> MLQQPTGGYTTLEQFAFTIRNDGTNATPTQFLQLLSWEATENELVKKTIPTPETHLPSARNVPGNVYIEDAITQAL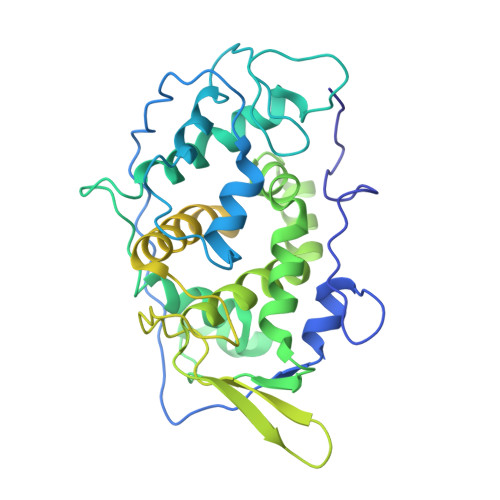FGISAQNVNAHGYFSRLSALALPNTSARLGLDGVIYNSETINIPFYDPAAVANFAATYAKLGNASTPRYRADMIDIYAHVGLELAGTDAERAAGVMPVKRAKFDSWEGSLISLSRDVVNWKILAFLIDLCSLEGEALRAFKTRNRDVFRMMLFIMSTAVAANVVNRKVTKRVDRVLEYIGVNSMRTAGRTATITYDLSRHEFAAKFLQLTFTRWNAASAMIRSMPDMHTPRTSITPAGENALVRHNRYMTENFKGLSPIALAQKKHEMMLHTHEIHSMDIDGSIKNMVERETVNKMNEIDAMNTAPWTEEFAEVEPTTVYERHQIGTDPEQTQLISQDAAVIVHQASSDVDENEYGNSVSELTIDTQSDSVL>FEEFNGKPDSLFFTDGQRRIDFILVYEDESKKENNKKGTNEKQKRKRQAYESNLICHGLQLEATRSVSDDKLVFVKVHAPWEVLCYYAEIMHIKLPLKPNDLKTRSPFGNLNWFTKVLRVNESVIKPEQEFFTAPFEKSRMNDFYILDRDSFFNPATRSRIVYFILSRVKYQVMNNVNKFGINRLVSSGIYKAAFPLHDCRFNYESEDISCPSERYLLYREWAHPRSIYKKQPLDLIRKYYGEKIGIYFAWLGYYTQMLLLAAVVGVACFLYGYLDQDNCTWSKEVCDPDIGGQILMCPQCDRLCPFWRLNITCESSKKLCIFDSFGTLIFAVFMGVWVTLFLEFWKRRQAELEYEWDTVELQQEEQARPEYEAQCNHVVINEITQEEERIPFTTCGKCIRVTLCASAVFFWILLIIASVIGIIVYRLSVFIVFSTTLPKNPNGTDPIQKYLTPQMATSITASIISFIIIMILNTIYEKVAIMITNFELPRTQTDYENSLTMKMFLFQFVNYYSSCFYIAFFKGKFVGYPGDPVYLLGKYRSEECDPGGCLLELTTQLTIIMGGKAIWNNIQEVLLPWVMNLIGRYKRVSGSEKITPRWEQDYHLQPMGKLGLFYEYLEMIIQFGFVTLFVASFPLAPLLALVNNILEIRVDAWKLTTQFRRMVPEKAQDIGAWQPIMQGIAILAVVTNAMIIAFTSDMIPRLVYYWSFSIPPYGDHTYYTMDGYINNTLSVFNITDFKNTDKENPYIGLGNYTLCRYRDFRNPPGHPQEYKHNIYYWHVIAAKLAFIIVMEHIIYSVKFFISYAIPDVSKITKSKIKRE[2x]

The dual functions of TMEM16F as Ca2+-activated ion channel and lipid scramblase raise intriguing questions regarding their molecular basis. TMEM16 proteins form dimers; each subunit comprises 10 transmembrane helices (TMs) and contains its own ion conduction pore surrounded by TM3-TM7. Ca2+-dependent activation involves direct binding of Ca2+ ions to two contiguous Ca2+-binding sites formed by TM6-TM8. Here, we report evidence for a lipid scrambling pathway along a groove harboring a lipid trail outside the ion permeation pore.

Here too we identified 3 distinct classes that closely resemble the 3 states observed in our drug-free sample. However, lipid densities along the membrane-facing surface of each monomer are absent. Instead, in all three classes we found a strong oval-shaped density in the same hydrophobic groove identified as the drug binding site in our niclosamide-supplemented dataset. Our structures show that both modulators replace the lipids found in this pocket in our drug-free sample. With both modulators directly contacting the extracellular-proximal end of TM6, our mutagenesis studies suggest that residues on this helix are critical for drug binding. We thus speculate that, by binding to the upper part of TM6, these modulators may simultaneously lock the ion conduction pore as well as the gating element in a closed configuration. The inhibitory effect of both antagonists was significantly decreased by all the mutations, confirming that these residues are important for binding these inhibitors.> GKAGKKLHYKQIVWVKLGNYRWWPAEICNPRS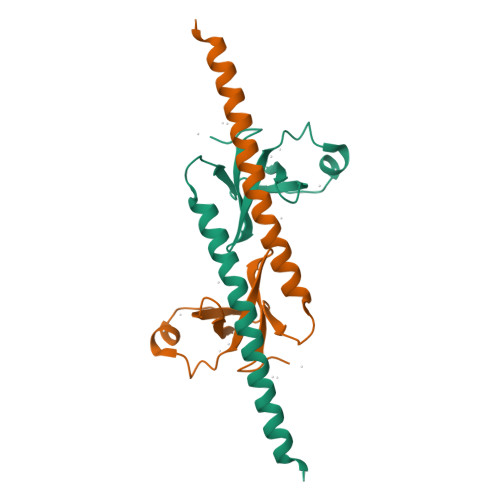VPLNIQGLKHDLGDFPVFFFGSHDYYWVHQGRVFPYVEGDKSFAEGQTSINKTFKKALEEAAKRFQELKAQRESKEALEIE>MSLLTEVETYVLSIIPSGPLKAEIAQRLEDVFAGKNTDLEVLMEWLK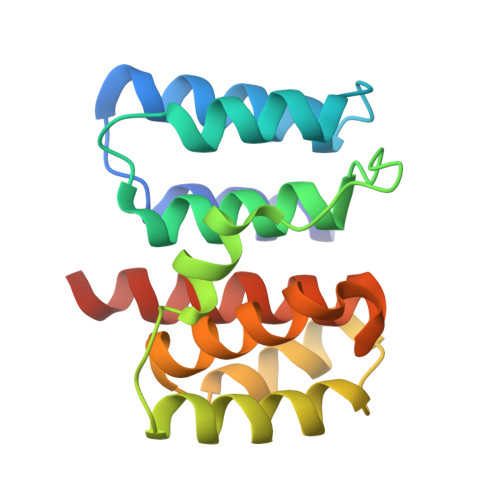TRPILSPLTKGILGFVFTLTVPSERGLQRRRFVQNALNGNGDPNNMDKAVKLYRKLKREITFHGAKEISLSYSAGALASCMGLIYNRMGAVTTEVAFGLVCATCEQIADSQHRSHRQ[2x]>MSKRPNFLVIVADDLGFSDIGTFGGEIATPNLDALAIAGLRLTDFHTASAASPTRSMLLTGTDHHIAGIGTMAEALTPELEGKPGYEGHLNERVVALPELLREAGYQTLMAGKWHLGLKPEQTPHARGFERSFALLPGAANHYGFEPPYDESTPRILKGTPALYVEDERYLDTLPEGFYSSDAFGDKLLQYLKERDQSRPFFAYLPFSAPHWPLQAPREIVEKYRGRYDAGPEALRQERLARLKELGLVEADVEAHPVLALTREWEALEDEERAKSARAMEVYAAMVERMDWNIGRVVDYLRRQGELDNTFVLFMSDNGAEGALLEAFPKF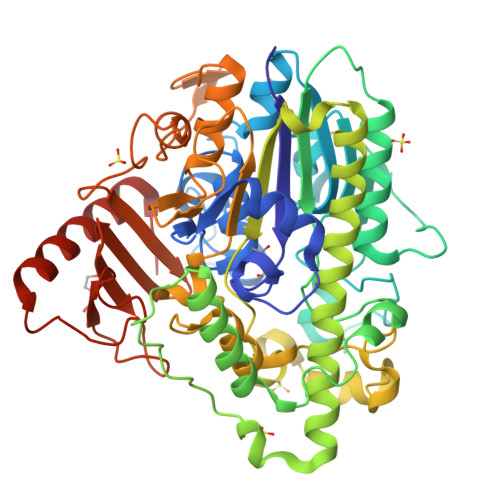GPDLLDFLDRHYDNSLENIGRANSYVWYGPRWAQAATAPSRLYKAFTTQGGIRVPALVRYPRLSRQGAISHAFATVMDVTPTLLDLAGVRHPGKRWRGREIAEPRGRSWLGWLSGETEAAHDENTVTGWGLFGMRAIRQGDWKAVYLPAPVGPATWQLYDLARDPGEIHDLADSQPGKLAELIEHWKRYVSDTGVVEGASPFLVR[2x]> MSQEALKAPVV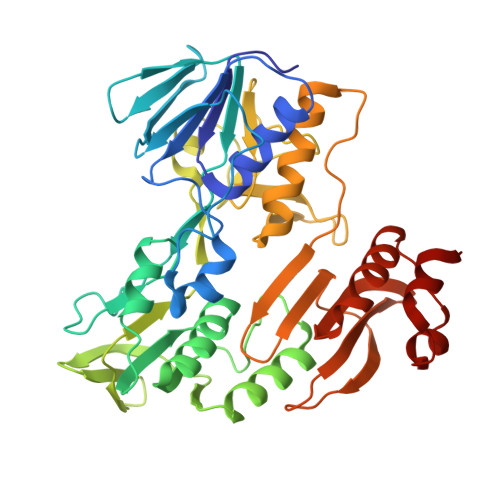VLGAGLASVSFVAELRQAGYQGLITVVGDEAERPYDRPPLSKDFMAHGDAEKIRLDCKRAPEVEWLLGVTAQSFDPQAHTVALSDGRTLPYGTLVLATGAAPRALPTLQGATMPVHTLRTLEDARRIQAGLRPQSRLLIVGGGVIGLELAATARTAGVHVSLVETQPRLMSRAAPATLADFVARYHAAQGVDLRFERSVTGSVDGVVLLDDGTRIAADMVVVGIGVLANDALARAAGLACDDGIFVDAYGRTTCPDVYALGDVTRQRNPLSGRFERIETWSNAQNQGIAVARHLVDPTAPGYAELPWYWSDQGALRIQVAGLASGDEEIVRGEVSLDAPKFTLIELQKGRIVGATCVNNARDFAPLRRLLAVGAKPDRAALADPATDLRKLAAAVAA> DSTTPGYTVVKNDWKKAVKQLQDGLKNKTISTIKVSFNGNSVGEVTPASSGAKKADRDAAAEKLYNLVNTQLDKLGDGDYVDFEVTYNLATQIITKAEAEAVLTKLQQYNDKVLINSATDTVKGMVSDTQVDSKNVAANPLKVSDMYTIPSAITGSDDSGYSIAKPTEKTTSLLYGTVGDATAGKAITVDTASNEAFAGNGKVIDYNKSFKATVQGDGTVKTSGVVLKDASDMAATGTIKVRVTSAKEESIDVDSSSYISAENLAKKYVFNPKEVSEAYNAIVALQN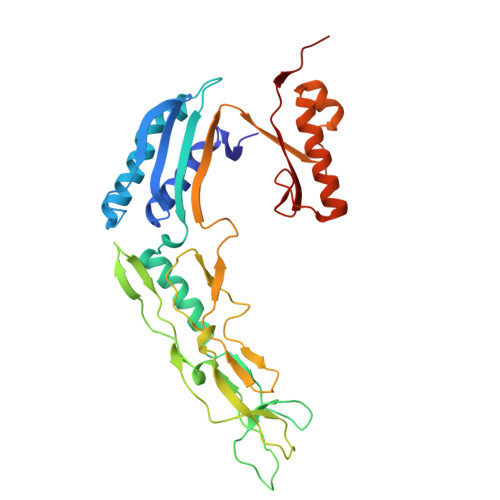DGIESDLVQLVNGKYQVIFYPEGKRLETKS>[3x]SVLQ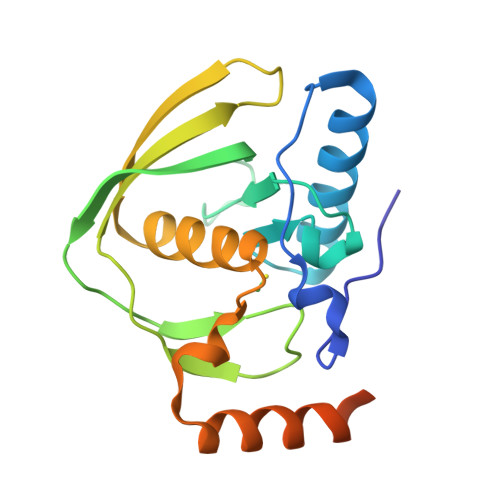VLHIPDERLRKVAKPVEEVNAEIQRIVDDMFETMYAEEGIGLAATQVDIHQRIIVIDVSENRDERLVLINPELLEKSGETGIEEGCLSIPEQRALVPRAEKVKIRALDRDGKPFELEADGLLAICIQHEMDHLVGKLFMDYLSPLKQQRIRQKVEKLDRLKARASSSVDKLAAALEHHHHHH> MGIDINTKIFNSVAEVFQKAQGSYAGHRKHIAVLKKIQSKAVEQGYEDAFNFWFDKLVTKILPLKKNEIIGDRIVKLVAAFIASLERELILAKKQNYKLTNDEEGIFSRFVDQFIRHVLRGVESPDKNVRFRVLQLLAVIMDNIGEIDESLFNLLILSLNKRIYDREPTVRIQAVFCLTKFQDEEQTEHLTELSDNEENFEATRTLVASIQNDPSAEVRRAAMLNLINDNNTRPYILERARDVNIVNRRLVYSRILKSMGRKCFDDIEPHIFDQLIEWGLEDRELSVRNACKRLIAHDWLNALDGDLIELLEKLDVSRSSVCVKAIEALFQSRPDILSKIKFPESIWKDFTVEIAFLFRAIYLYCLDNNITEMLEENFPEASKLSEHLNHYILLRYHHNDISNDSQSHFDYNTLEFIIEQLSIAAERYDYSDEVGRRSMLTVVRNMLALTTLSEPLIKIGIRVMKSLSINEKDFVTMAIEIINDIRDDDIEKQESESDIINNLPPEKEASSATIVLCLTRSSYMLELVNTPLTENILIASLMDTLITPAVRNTAPNIRELGVKNLGLCCLLDVKLAIDNMYILGMCVSKGNASLKYIALQVIVDIFSVHGNTVVDGEGKVDSISLHKIFYKVLKNNGLPECQVIAAEGLCKLFLADVFTDDDLFETLVLSYFSPINSSNEALVQAFAFCIPVYCFSHPAHQQRMSRTAADILLRLCVLWDDLQSSVIPEVDREAMLKPNIIFQQLLFWTDPRNLVNQTGSTKKDTVQLTFLIDVLKIYAQIEKKEIKKMIITNINAIFLSSEQDYSTLKELLEYSDDIAENDNLDNVSKNALDKLRNNLNSLIEEINERSETQTKDENNTANDQYSSILGN;> GPLGHMSIFEKDLMAYFDENLNRNWRGREHWKVRNFKKANLVNKESDLLEETRTTIGDTTDKNTTDDKSMDTKKKHKQKKVLEIDFFKTDDSFEDKVFASKGRTKIDMPIKNRKNDTHYLLPDDFHFSTDRITRLFIKPGQKMSLFSHRKHT

Condensin protein complexes coordinate the formation of mitotic chromosomes and thereby ensure the successful segregation of replicated genomes. Here, we identify a direct DNA-binding site in the eukaryotic condensin complex, which is formed by its Ycg1Cnd3 HEAT-repeat and Brn1Cnd2 kleisin subunits. A peptide loop of the kleisin subunit encircles the bound DNA and, like a safety belt, prevents its dissociation. Firm closure of the kleisin loop around DNA is essential for the association of condensin complexes with chromosomes and their DNA-stimulated ATPase activity.

Whereas several basic residues of Ycg1 and Brn1 directly contact the DNA phosphate backbone, several other residues are oriented toward the DNA but are too far away to make direct electrostatic interactions. As a result, the Ycg1–Brn1 groove might allow some degree of flexibility in accommodating the DNA double helix. This notion is further supported by a second crystal structure of Ycg1–Brn1 in complex with the same 18-bp DNA substrate, which crystallized with slightly different unit cell dimensions. Compared to the first DNA co-structure, the C-terminal Ycg1 shoulder is slightly translocated, and as a consequence, the contacts between this part of Ycg1–Brn1 and DNA differ considerably from the other crystal form. The conformational flexibility in the contacts with DNA revealed by two Ycg1–Brn1–DNA crystal forms and the low binding affinity to short linear DNA fragments suggest that the positively charged groove alone can only weakly interact with DNA duplexes. The facts that DNA contacts are made exclusively with the phosphate backbone and are conformationally adaptable provide the HEAT-repeat and kleisin subunits of condensin with the means to bind DNA independent of sequence or specific local structure, which contrasts sharply with the conventional concept of protein-DNA recognition (Rohs et al., 2010). Even in the co-crystal structures of Sc Ycg1–Brn1 with DNA, 43 residues of the linker that connects the α1 and α2 segments of Brn1 remained disordered. The trajectories of the visible residues that flank the linker, however, indicate that the path of the connecting peptide leads over the bound DNA helix.Fragaceatoxin C (FraC)11 is a potent haemolysin of the family of actinoporins, defined as a group of ~20 kDa protein toxins produced by sea anemones. Actinoporins are classified as α-helical PFT (α-PFT) because the transmembrane pore is predicted to form an α-helical barrel. The lytic activity of actinoporins on biological membranes is enhanced by the lipid sphingomyelin (SM) and by lipid-phase coexistence. Here we reveal structures of FraC corresponding to four different stages of its activation route, namely the water-soluble form, the lipid-bound form, an assembly intermediate and the transmembrane pore.

To examine the lipid-bound conformation, we determined three independent crystal structures of FraC in complex with the water-soluble lipid 1,2-dihexanoyl-sn-glycero-3-phosphocholine (DHPC) at resolutions ranging from 1.6 to 2.3 Å. Remarkably, up to four lipid molecules are bound to a single protein chain. The molecules of DHPC bound to each molecule of FraC lie on a common plane, resembling the surface of a membrane. Although multiple molecules of DHPC bind to FraC, the toxin remains monomeric and its overall structure is virtually unchanged with respect to that of the water-soluble form (rmsd=0.37±0.10 Å). The examination of the structure in three different crystal forms reveals two well-conserved lipid-binding pockets, suggesting they are the primary sites during the initial adhesion of FraC to membranes. These two pockets overlap with those of lipids L2 and L3 seen in the structure of the transmembrane pore, and establish comparable non-covalent interactions with the lipids. In contrast, no evidence of the L1 lipid is found because the protein remains monomeric and, therefore, lacks a second protein chain contributing half of the binding site of L1. FraC–lipid interactions occur mainly at the headgroup region of the lipids. Because the headgroups of SM and DHPC are identical, that is, phosphorylcholine (POC), the crystal structures explain the targeting of actinoporins towards synthetic membranes containing these two types of lipids.

>SADVAGAVIDGAGLGFDVLKTVLEALGNVKRKIAVGIDNESGKTWTAMNTYFRSGTSDIVLPHKVAHGKALLYNGQKNRGPVATGVVGVIAYSMSDGNTLAVLFSVPYDYNWYSNWWNVRVYKGQKRADQRMYEELYYHRSPFRGDNGWHSRGLGYGLKSRGFMNSSGHAILEIHVTKA[6x]> MKVTKVGGISHKKYTSEGRLVKSESEENRTDERLSALLNMRLDMYIKNPSSTETKENQKRIGKLKKFFSNKMVYLKDNTLSLKNGKKENIDREYSETDILESDVRDKKNFAVLKKIYLNENVNSEELEVFRNDIKKKLNKINSLKYSFEKNKANYQKINENNIEKVEGKSKRNIIYDYYRESAKRDAYVSNVKEAFDKLYKEEDIAKLVLEIENLTKLEKYKIREFYHEIIGRKNDKENFAKIIYEEIQNVNNMKELIEKVPDMSELKKSQVFYKYYLDKEELNDKNIKYAFCHFVEIEMSQLLKNYVYKRLSNISNDKIKRIFEYQNLKKLIENKLLNKLDTYVRNCGKYNYYLQDGEIATSDFIARNRQNEAFLRNIIGVSSVAYFSLRNILETENENDITGRMRGKTVKNNKGEEKYVSGEVDKIYNENKKNEVKENLKMFYSYDFNMDNKNEIEDFFANIDEAISSIRHGIVHFNLELEGKDIFAFKNIAPSEISKKMFQNEINEKKLKLKIFRQLNSANVFRYLEKYKILNYLKRTRFEFVNKNIPFVPSFTKLYSRIDDLKNSLGIYWKTPKTNDDN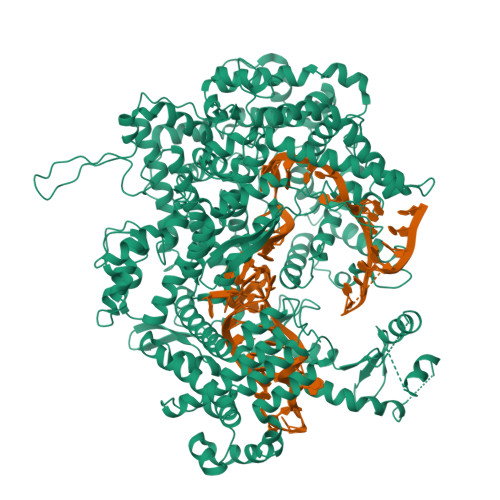KTKEIIDAQIYLLKNIYYGEFLNYFMSNNGNFFEISKEIIELNKNDKRNLKTGFYKLQKFEDIQEKIPKEYLANIQSLYMINAGNQDEEEKDTYIDFIQKIFLKGFMTYLANNGRLSLIYIGSDEETNTSLAEKKQEFDKFLKKYEQNNNIKIPYEINEFLREIKLGNILKYTERLNMFYLILKLLNHKELTNLKGSLEKYQSANKEEAFSDQLELINLLNLDNNRVTEDFELEADEIGKFLDFNGNKVKDNKELKKFDTNKIYFDGENIIKHRAFYNIKKYGMLNLLEKIADKAGYKISIEELKKYSNKKNEIEKNHKMQENLHRKYARPRKDEKFTDEDYESYKQAIENIEEYTHLKNKVEFNELNLLQGLLLRILHRLVGYTSIWERDLRFRLKGEFPENQYIEEIFNFENKKNVKYKGGQIVEKYIKFYKELHQNDEVKINKYSSANIKVLKQEKKDLYIANYIAAFNYIPHAEISLLEVLENLRKLLSYDRKLKNAVMKSVVDILKEYGFVATFKIGADKKIGIQTLESEKIVHLKNLKKKKLMTDRNSEELCKLVKIMFEYKMEEKKSEN> LRDVILVSKDIPEQLCDALFFYTSHNPKDYADAFAVRQKFDRNLQTGKQFKFETVCGLFLLKGVDKITPGVPAKVLKATSKLADLEDIFGVSPFARKYRELLK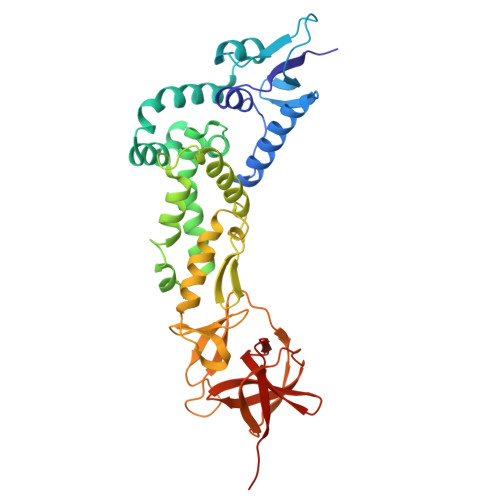TACQWSLTVETLDARALTLDEIFDPTEILWLQVAAKIQVSAMAMRRLVGEVTAKVMDALGSNMSALFQIFKQQIVRIFQAALAIFENVSELPQRIAALKMAFAKCAKSITVVVMERTLVVREFAGTCLASINGAVAKFFEELPNGFMGAKIFTTFAFFREAAVKIVDNIPNAPRGTKGFEVVGNAKGTQVVVRGMRNDLTLLDQKAEIPVESEGWSAILGGHLCYVFKSGDRFYAAPLSGNFALHDVHCCERVVCL> GSHMDASVMSTTYALSAAQTEIWLAQQLYPDSPVYNIAQYTVIEGVIEPAVFEAALRQVIDEADTLRLQFIDSDDGLRQRIGTPAWSMPVLDLTAQADPQAAAQAWMRADYQQPVNLTQGPLFCYALLKVAPAQWMWYQRYHVIMMDGYGAYLIAQRVAYVYSALCEGTTPAECDFGSILQLLESDAQYQISAQRAQDEAYWLKHCANWSEPATLASRSAPVLQQRLRQTTYLAIQALGDTAPDARRLAQFMTAAMAAYLYRFTGEQDVVLGLPVKVRFGADRHIPGMKSNTLPLRLTMRPGMNLSSLMQQAAQEMQSGLRHQRYPSEALRRQLGMPSGQRLFGTTVNVMPFDLDLSFGGYSATNHNLLNGPAEDLMLGVYWTPGSHQLRIDFDANPACYTPEGLGAHQRRFIRFMQVLAADATQPIDSIDLLD

Nonribosomal peptide synthetases (NRPSs) are multimodular enzymes that catalyze the biosynthesis of diverse peptides with a wide variety of activities. The incorporation of an acyl into peptidyl backbone is usually implemented by a starter condensation (Cs) domain, normally located at the beginning of the initial NRPS module, via the formation of an amide bond to the α-amino group of the first amino acid residue, a process also known as lipoinitiation. Genome mining of two Cs domain-embedded cryptic NRPS biosynthetic gene clusters, rzmA and holA, in the bacterium P. rhizoxinica HKI 454 resulted in the discovery of two distinct types of lipopeptides, cyclic rhizomide A (1) containing an uncommon acetyl chain (C2) and linear holrhizin A (2) harboring a medium octanoyl (C8) chain. Similar to other C domain structures reported previously, RzmA-Cs adopts a “V-shaped” configuration and consists of two subdomains (N- and C-lobes) each representing the chloramphenicol acetyltransferase (CAT) fold.

To diminish the reaction rate, we made an additional mutation on the second histidine of the “HHxxxDG” motif37 of RzmA-Cs R148A to create the double mutant H140V/R148A, which finally enabled us to obtain several crystals in the absence or presence of substrates. Then, we compared the C8-CoA-bound structures of H140V/R148A and R148A. Although their overall structures are quite similar, we noticed that the electron densities surrounding the C8 acyl chain (but not the CoA portion) are much worse in the H140V/R148A structure than in the R148A structure. These results indicate that the acyl chain of the substrate in the H140V/R148A structure is more flexible with H140 mutated to valine, again confirming the role of H140 in positioning the “donor” acyl-CoAs. Our co-complex structures of RzmA-Cs not only supported this conception, but also extended the positioning function of this histidine (H140) to the donor substrates, i.e., acyl-CoAs.> MEAGITGTWYNQLGSTFIVTAGADGALTGTYVTARGNAESRYVLTGRYDSAPATDGSGTALGWTVAWKNNYRNAHSATTWSGQYVGGAEARINTQWLLTSGTTEENAGYSTLVG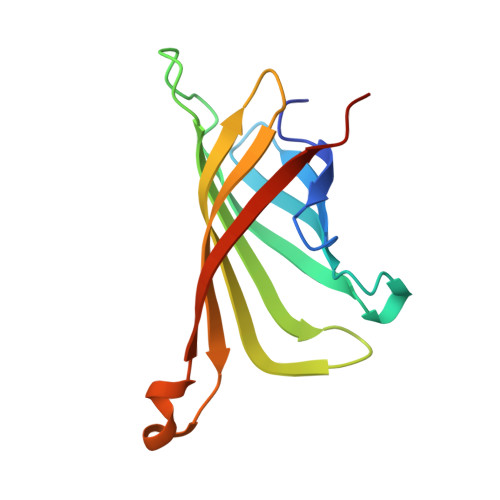HDTFTKVKPSAAS> K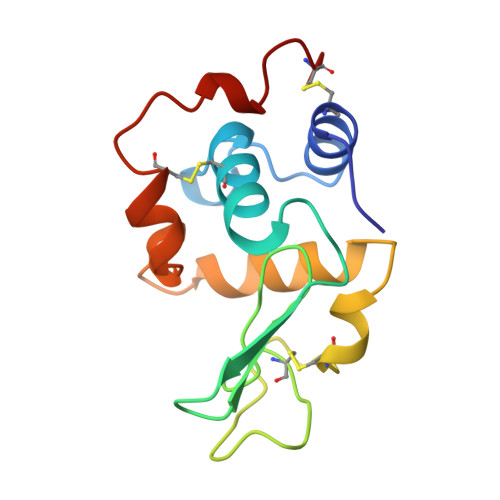VFERCELARTLKRLGMDGYRGISLANWMCLAKWESGYNTRATNYNAGDRSTDYGIFQINSRYWCNDGKTPGAVNAAHLSCSALLQDNIADAVAAAKRVVRDPQGIRAWVAWRNRCQNRDVRQYVQGCGA>SLEIPSKQIDYRDVFIEFLTTFKGNNNQNKYIERINELVAYRKKSLIIEFSDVLSFNENLAYEIINNTKIILPILEGALYDHILQLDPTYQRDIEKVHVRIVGIPRVIELRKIRSTDIGKLITIDGILVKVTPVKERIYKATYKHIHPDCMQEFEWPEDEEMPEVLEMPTICPKCGKPGQFRLIPEKTKLIDWQKAVIQERPEEVPSGQLPRQLEIILEDDLVDSARPGDRVKVTGILDIKQDSPVKRGSRAVFDIYMKVSSIEVSGGSGGSSEEDEKKIKDLAKDPWIRDRIISSIAPSIYGHWELKEALALALFGGVPKVLEDTRIRGDIHILIIGDPGTAKSQMLQFISRVAPRAVYTTGKGSTAAGLTAAVVREKGTGEYYLEAGALVLADGGIAVIDEIDKMRDEDRVAIHEAMEQQTVSIAKAGIVAKLNARAAVIAAGNPKFGRYISERPVSDNINLPPTILSRFDLIFILKDQPGEQDRELANYILDVHSGKSTKNIIDIDTLRKYIAYARKYVTPKITSEAKNLITDFFVEMRKKSSETPDSPILITPRQLEALIRISEAYAKMALKAEVTREDAERAINIMRLFLESVGVDMESGKIDID[6x]

A six-subunit ATPase ring forms the central hub of the replication forks in all domains of life. This ring performs a helicase function to separate the two complementary DNA strands to be replicated and drives the replication machinery along the DNA. The helicase/ATPase rings of eukaryotes and archaea consist of six minichromosome maintenance (MCM) proteins. The MCM rings of archaeal organisms, such as Saccharolobus solfataricus, form a homohexameric ring.

To examine the mechanism of DNA translocation by the MCM hexameric helicase, we determined cryo-EM structures of a protein construct of the MCM protein from the archaeal organism Saccharolobus solfataricus (SsoMCM) in complex with the ATP analog ADP-BeF3, magnesium, and oligonucleotide. In attempting to reveal different aspects of DNA manipulation by the MCM helicase, cryo-EM structures were determined with three different oligonucleotides of different lengths and potential for secondary structure. Despite the differences of the oligonucleotides used for complex formation, each sample showed highly similar behavior with two distinct structural classes. The first class of structure is well-structured throughout and binds a very well-ordered segment of 11 nucleotides of ssDNA within the central channel at the ATPase tier. The ATPase tier is not 6-fold symmetric because the subunits form a helical “staircase” that binds encircled ssDNA. The sixth ATPase domain (red) interacts with ssDNA at the at the bottom of the staircase with just one hairpin. This subunit also loosely interacts with DNA at the top of the staircase. Specifically, transformation of class 1 with six subunits engaged to DNA to class 2 with five subunits engaged illustrates a dissociation of one subunit from DNA.> MENVAEPTVASVSKRIMHNAYYYDKDAKRVGTDSVKRYNSVSVLPNTTTINGKTYYQVVENGKAVDKYINAANIDGTKRTLKHNAYVYASSKKRANKVVLKKGEVVTTYGASYTFKNGQKYYKIGDNTDKTYVKVANFRLEHHHHH

S-layer proteins (SLPs) are self-assembling, crystalline proteins coating the cell surfaces of many prokaryotes. We determined the atomic resolution structures of all functional domains (I-III from N- to C-termini) present in the three S-layer proteins SlpA_ac, SlpX_ac, and SlpA_amy. The Lactobacillus S-layers are anchored to the cell wall through interaction with teichoic acids (TA), either lipoteichoic acid (LTA) or wall teichoic acid (WTA).

The SlpA protein (~46 kDa) is the main structural component of Lactobacillus acidophilus ATCC 4356 S-layer, built of two domains. The N-terminal region is involved in the self-assembly of the S-layer, whereas the C-terminal part is involved in the attachment to the cell wall. The amino acid sequence of the C-terminal SlpA_III domain is sequentially conserved among Lactobacillus. It consists of two adjacent repeats of the “SlpA-motif,” the “Surface layer protein A motif/domain” (InterPro: IPR024968). This domain is involved in the binding to TAs (teichoic acid binding domain; TAB domain), one of the components of the bacterial cell wall. The crystal structures of the TAB domains (SlpA_ac_III, SlpA_amy_III, and SlpX_ac_III) reveal high structural similarities. The general structure of the TAB domain consists of two cell wall binding motifs (SlpA_motif) which are connected by a short linker and arranged as an internal homodimer. Mapping of the surface charges indicates a large, highly positively charged region within the interface of the two motifs that extends to the C-terminal part of the protein. The four residues observed in the vicinity of phosphates are conserved with the proposed binding motif of YxY….KxxN. SlpA_III, the teichoic acid binding domain, is not involved in the self-assembly and protrudes inward to the bacterial cell.>[2x]MGSSHHHHHHSSENLYFQGHSEEAEVGISASTNIPGAQYPQILSGNRVLFRIKAPDAKRVQVDLGKKYDMVREEEGSWAITTDPIVEGFHYYSILIDGVAVCDPASRTFYGMSRMASGIEIPEEGVD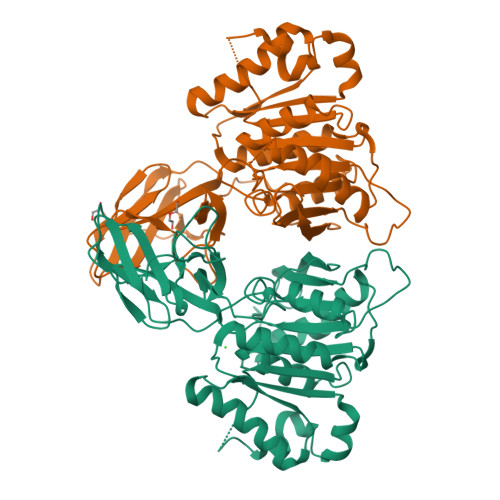YYNLKNVPHGQIRQIRYFSDVTKAWRRAFVYTPAGYDANTSQRYPVLYLQHGGGEDETGWPNQGKMDAIIDNLIAEGKAKPMIVVMDNGYAVDPSASSANSPQGLRGLFQNSALEKVFINEIIPLVDKEFRTIADRDHRAMAGLSMGGFQAFQIAMTNLDKFAYVGGFSGGGIIEQGGDFSKMYNNVWSDVDTFNKRVKLIYLSIGTAEPTNMYQTVNNFHKEFEKAGIKHVYYESPGTSHEWLTWRRSLNQFAELLFK>TYCVAMRLSSGLAFASDSRTNAGVDHISTFRKLHLFQQPGERTLVVQSAGNLATTQSIVSLLQRRCLDPEQTNLMNVASMYEAATLLGETVREVINRDSGAQQNSHGTDFNCNLLLGGQIKGEGLRLFHIYPQGNFIEATQDTPYFQIGESKYGKPIIDRVLSYDTPLDQAMQCALISMDSTLRSNLSVGLPLDVMIYPLDSFSTEQQYRITEDHPYFMMIRKGWGEGLVSIFAQLPGLKLGRLEHH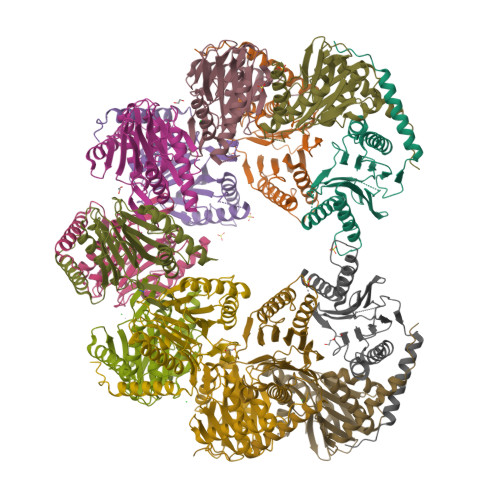HHHH[28x]> HHAADYVLYKDATKPVEDRVADLLGRMTLAEKIGQMTQIERLVATPDVLRDNFIGSLLSGGGSVPRKGATAKEWQDMVDGFQKACMSTRLGIPMIYGIDAVHGQNNVYGATIFPHNVGLGATRDPYLVKRIGEATALEVRATGIQYAFAPCIAVCRDPRWGRCYESYSEDRRIVQSMTELIPGLQGDVPKDFTSGMPFVAGKNKVAACAKHFVGDGGTVDGINENNTIINREGLMNIHMPAYKNAMDKGVSTVMISYSSWNGVKMHANQDLVTGYLKDTLKFKGFVISDAEGIDRITTPAGSDYSYSVKASILAGLDMIMVPNKYQQFISILTGHVNGGVIPMSRIDDAVTRILRVKFTMGLFENPYADPAMAEQLGKQEHRDLAREAARKSLVLLKNGKTSTDAPLLPLPKKAPKILVAGSHADNLGYQCGGWTIEWQGDTGRTTVGTTILEAVKAAVDPSTVVVFAENPDAEFVKSGGFSYAIVAVGEHPYTETKGDNLNLTIPEPGLSTVQAVCGG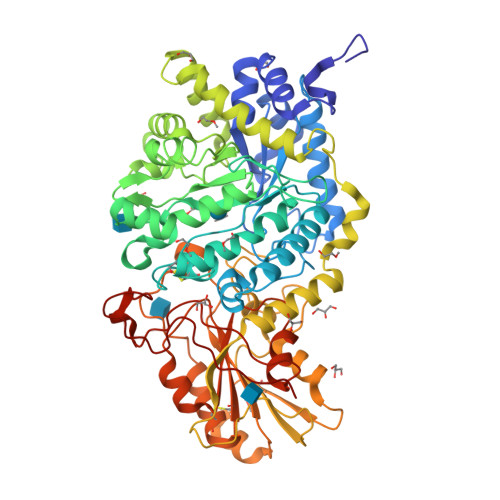VRCATVLISGRPVVVQPLLAASDALVAAWLPGSEGQGVTDALFGDFGFTGRLPRTWFKSVDQLPMNVGDAHYDPLFRLGYGLTTNATKKY> MREAIIKRAAKELKEGMYVNLGIGLPTLVANEVSGMNIVFQSENGLLGIGAYPLEGSVDADLINAGKETITVVPGASFFNSADSFAMIRGGHID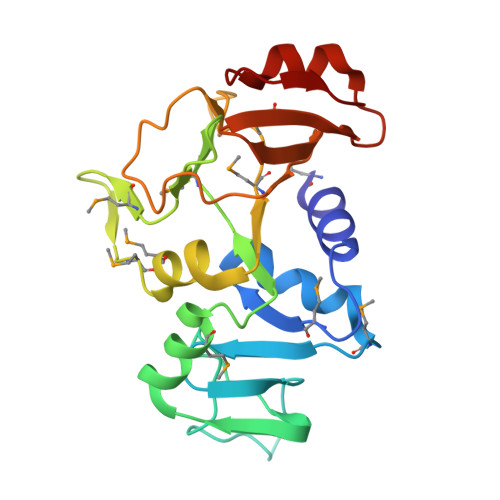LAILGGMEVSQNGDLANWMIPKKLIKGMGGAMDLVHGAKKVIVIMEHCNKYGESKVKKECSLPLTGKGVVHQLITDLAVFEFSNNAMKLVELQEGVSLDQVKEKTEAEFEVRL> MDEFEMIKRNTSEIISEEELREVLKKDEKSALIGFEPSGKIHLGHYLQIKKMIDLQNAGFDIIIILADLGAYLNQKGELDEIRKIGDYNKKVFEAMGLKAKYVYGSEILLDKDGTLNVYRLALKTTLKRARRSMELIAREDENPKVAEVIYPIMQVNSIHYMGVDVAVGGMEQRKIHMLARELLPKKVVCIHNPVLTGLDGEGKMSSSKGNFIAVDDSPEEIRAKIKKAYCPAGVVEGNPIMEIAKYFLEYPLTIKRPEKFGGDLTVNSYEELESLFKNKELHPMDLKNAVAEELIKILEPI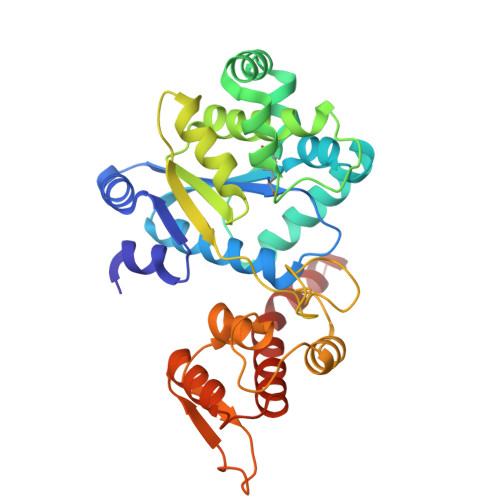RKRLAHHHHHH> MAHHHHHHVDDDDKTDPR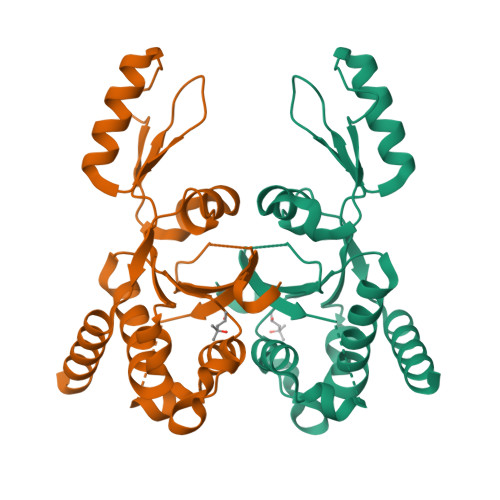KSELYVVEGDSAGGSAKSGRDSMFQAILPLRGKIINVEKARIDRVLKNTEVQAIITALGTGIHDEFDIGKLRYHKIVLMADADVDGQHISTLLLTLLFRFMRPLIENGHVFLAQPPLYKLKWQRSDPEFAYSDRERDGLLEAGLKAGKKINKEDGIQRYKGLGEMDAKELWETTMDPSVRVLRQVTLDDAAAADELFSILMGEDVDARRSFITRNAKDVRFLDV2-aminopyrimido[4,5-d]pyrimidin-4(3H)-one 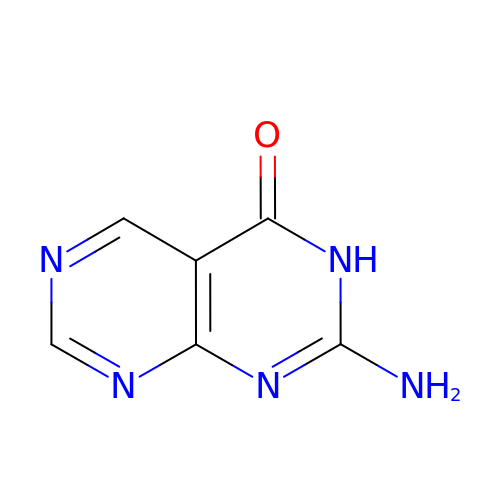| C6 H5 N5 O | HHOGMIYMABYION-UHFFFAOYSA-N> HGFVQNIVIDGKNYGGYLVNQYPYMSNPPEVIAWSTTATDLGFVDGTGYQTPDIICHRGAKPGALTAPVSPGGTVELQWTPWPDSHHGPVINYLAPCNGDCSTVDKTQLEFFKIAESGLINDDNPPGIWASDNLIAANNSWTVTIPTTIAPGNYVLRHEIIALHSAQNQDGAQNYPQCINLQ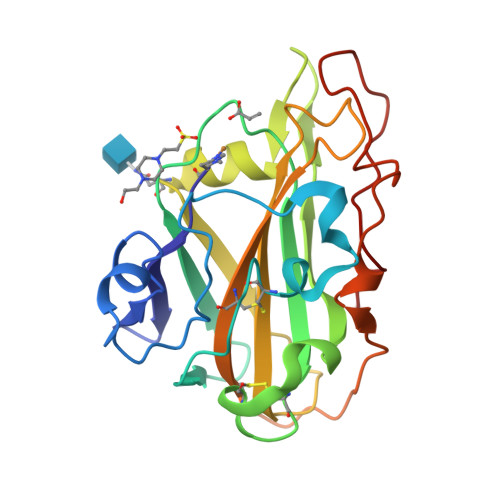VTGGGSDNPAGTLGTALYHDTDPGILINIYQKLSSYIIPGPPLYTG1-{5-chloro-2-[(3R)-pyrrolidin-3-yloxy]phenyl}-3-(5-cyanopyrazin-2-yl)urea | C16 H15 Cl N6 O2 | 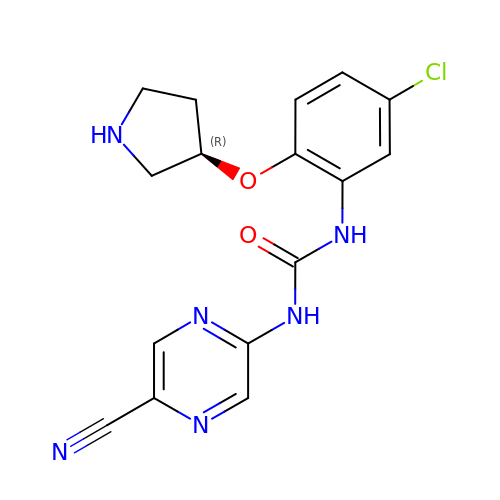XWBVWQBBHHJLKT-GFCCVEGCSA-N> MSETTMYTVSSSPHIRAKDTTQSIMRDVVIALLPATIAGVYFFKLQGLLVILASVLSCVVAEYIWQKASKKKVTVGD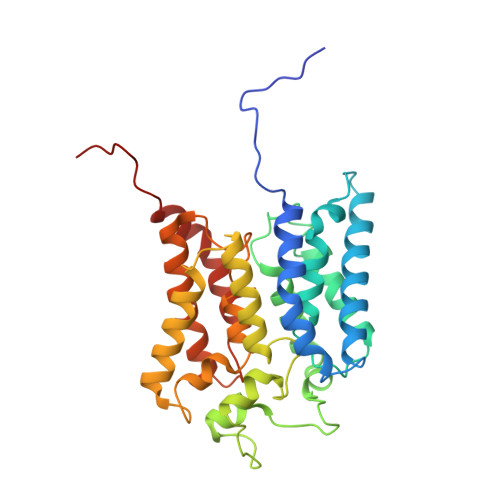YSAVVTGLLLAFNVPASIPLWIPVVGGFFAIIVVKQFFGGLGQNIVNPALAARAFLLASWPVQMTSWTLDGVTTATPLAILKGNEATGAAAPDLMSVFIGHVGGCIGETSALALLIGGAYLFYKHIIDWRIPVSFIGTTFIFTAIAGRGSSPVYELFAGGLMLGAIFMATDYATSPITPLGRIIFGVGCGVITSLIRIFGGYPEGVSYSILVMNLFVPLIERWTAPKIFGKVK> MAEHGESSEDRISEIDYEFLPELSALLGVDAFQVAKSQEEEEHKERMKMKKGFNSQMRSEAKRLKTFETYDTFRSWTPQEMAAAGFYHTGVKLGVQCFCCSLILFGNSLRKLPIERHKKLRPECEFLQGKDVGNIGKYDIRVKSPEKMLRGGKARYHEEEARLESFEDWPFYAHGTSPRVLSAAGFVFTGKRDTVQCFSCGGSLGNWEEGDDPWKEHAKWFPKCEFLQSKKSSEEIAQYIQSYEGFVHVTGEHFVKSWVRRELPMVSAYCNDSVFANEELRMDMFKDWPQESPVGVEALVRAGFFYTGKKDIVRCFSCGGCLEKWAEGDDPMEDHIKFFPECVFLQTLKSSAEVIPTLQSQYALPEATETTRESNHGDAAAVHSTVVDLGRSEAQWFQEARSLSEQLRDNYTKATFRHMNLPEVCSSLGTDHLLSCDVSIISKHISQPVQEALTIPEVFSNLNSVMCVEGETGSGKTTFLKRIAFLWASGCCPLLYRFQLVFYLSLSSITPDQGLANIICAQLLGAGGCISEVCLSSSIQQLQHQVLFLLDDYSGLASLPQALHTLITKNYLSRTCLLIAVHTNRVRDIRLYLGTSLEIQEFPFYNTVSVLRKFFSHDIICVEKLIIYFIDNKDLQGVYKTPLFVAAVCTDWIQNASAQDKFQDVTLFQSYMQYLSLKYKATAEPLQATVSSCGQLALTGLFSSCFEFNSDDLAEAGVDEDEKLTTLLMSKFTAQRLRPVYRFLGPLFQEFLAAVRLTELLSSDRQEDQDLGLYYLRQIDSPLKAINSFNIFLYYVSSHSSSKAAPTVVSHLLQLVDEKESLENMSENEDYMKLHPQTFLWFQFVRGLWLVSPESSSSFVSEHLLRLALIFAYESNTVAECSPFILQFLRGKTLALRVLNLQYFRDHPESLLLLRSLKVSINGNKMSSYVDYSFKTYFENLQPPAIDEEYTSAFEHISEWRRNFAQDEEIIKNYENIRPRALPDISEGYWKLSPKPCKIPKLEVQVNNTDAADQALLQVLMEVFSASQSIEFRLFNSSGFLESICPALELSKASVTKCSMSRLELSRAEQELLLTLPALQSLEVSETNQLPEQLFHNLHKFLGLKELCVRLDGKPDVLSVLPGEFPNLHHMEKLSIRTSTESDLSKLVKFIQNFPNLHVFHLKCDFLSNCESLMAVLASCKKLREIEFSGRCFEAMTFVNILPNFVSLKILNLKDQQFPDKETSEKFAQALGSLRNLEELLVPTGDGIHQVAKLIVRQCLQLPCLRVLTFHDILDDDSVIEIARAATSGGFQKLENLDISMNHKITEEGYRNFFQALDNLPNLQELNICRNIPGRIQVQATTVKALGQCVSRLPSLIRLHMLSWLLDEEDMKVINDVKERHPQSKRLIIFWKLIVPFSPVILE;>MNFIRNNRRALIQRMGLTVTKQICDDLFALNVLNNQEANVIYCEPLEQEAARKIIHMTMQKGSAACNLFLKSLENWDYFVYQDLTGQNLSYQVTEEDLNVLAQNLKDLYNSPAFLNFYPLGEDIDIIFNLEKTFTEPIMWKKDHRHHRVEQLTLGSLLEALKSPCLIEGESGKGKSTLLQRIAMLWASGGCRALKGFRLVFFIHLRSARGGLFETLYDQLLNIPDFISKPTFKALLLKLHKEVLFLLDGYNEFHPQNCPEIEALIKENHRFKNMVIVTTTTECLRHIRHVGALTAEVGDMTEDSAKDLIEAVLVPDQVERLWAQIQESRCLRNLMKTPLFVVITCAIQMGRQEFQAHTQTMLFQTFYDLLIQKNSHRYRGGASGDFARSLDYCGDLALEGVFAHKFDFEPEHGSSMNEDVLVTIGLLCKYTAQRLKPTYKFFHKSFQEYTAGRRLSSLLTSKEPEEVSKGNSYLNKMVSISDITSLYGNLLLYTCGSSTEATRAVMRHLAMVYQHGSLQGLSVTKRPLWRQESIQSLRNTTEQDVLKAINVNSFVECGINLFSESMSKSDLSQEFEAFFQGKSLYINSENIPDYLFDFFEYLPNCASALDFVKLDFYERATESQDKAEENVPGVHTEGPSETYIPPRAVSLFFNWKQEFKTLEVTLRDINKLNKQDIKYLGKIFSSATNLRLHIKRCAAMAGRLSSVLRTCKNMHTLMVEASPLTTDDEQYITSVTGLQNLSIHRLHTQQLPGGLIDSLGNLKNLERLILDDIRMNEEDAKNLAEGLRSLKKMRLLHLTHLSDIGEGMDYIVKSLSEESCDLQEMKLVACCLTANSVKVLAQNLHNLIKLSILDISENYLEKDGNEALQELIGRLGVLGELTTLMLPWCWDVHTSLPKLLKQLEGTPGLAKLGLKNWRLRDEEIKSLGEFLEMNPLRDLQQLDLAGHCVSSDGWLYFMNVFENLKQLVFFDFSTEEFLPDAALVRKLSQVLSKLTLLQEVKLTGWEFDDYDISAIKGTFKLVTA[2x];> MEQKLISEEDLNEMEQKLISEEDLNEMEQKLISEEDLNEMEQKLISEEDLNEMEQKLISEEDLNEMESLGDLTMEQKLISEEDLNSGRPAAMAQVINTNVASLTAQRNLGVSGNMMQTSIQRLSSGLRINSAKDDAAGLAISQRMTAQIRGMNQAVRNANDGISLAQVAEGAMQETTNILQRMRELSVQAANSTNNSSDRSSIQSEISQLKSELERIAQNTEFNGQRILDGSFSGASFQVGANSNQTINFSIGSTKASSLGGIATATGTEVAGAAAADITIAIGGGAATSINSSANFTGALNGQDATSAYAKAAAINDAGIGGLSVTASTSGTQAVGAIGGTAGDTYNLTINGVAIYTNLNVATALTNSDLRDAINGVSNQTGVVASLNGGNMTLTAADGRNITVTESGTGFTAGTDGLTVTGGAFDGALRGTLSISAVDTIAIGGTVANIGLSANISKDTVGIDSLDV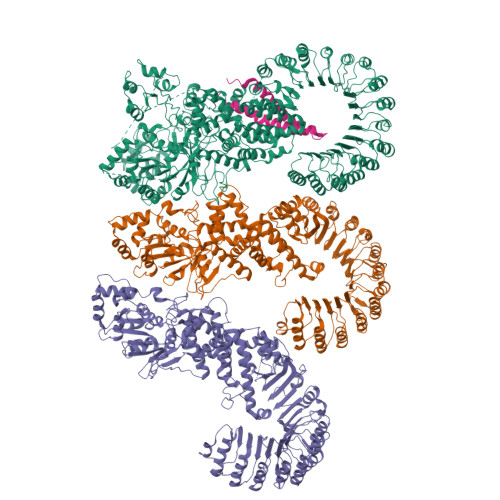STASGAQTAIKRIDAALNSVNSNRANMGALQNRFESTIANLQNVSDNLSAARSRIQDADYAAEMASLTKNQILQQAGTAMLAQANSLPQSVLSLLGR(2~{S})-4-methyl-~{N}-prop-2-enyl-2-[[(1~{S})-2,2,2-tris(fluoranyl)-1-[4-(4-methylsulfonylphenyl)phenyl]ethyl]amino]pentanamide | C24 H29 F3 N2 O3 S | 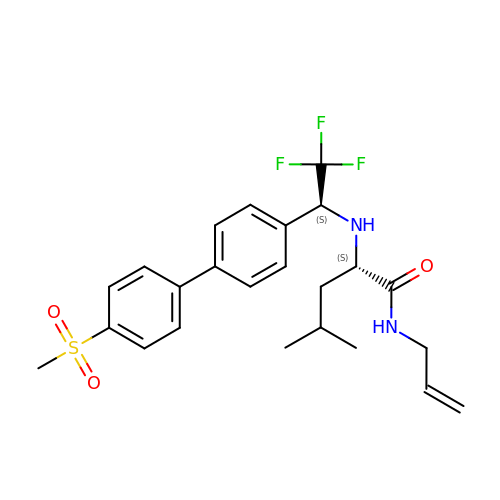HWJULRRDJXNVSU-VXKWHMMOSA-N> MTENIEAVMSDFWSNPADHFRPNLKALTLYAERQHYVDRWLHVKERWLAPWYLPWWSPLFQLGTWYSQRSRNLFLVENHLSYRPYKFRRNDEDRNNP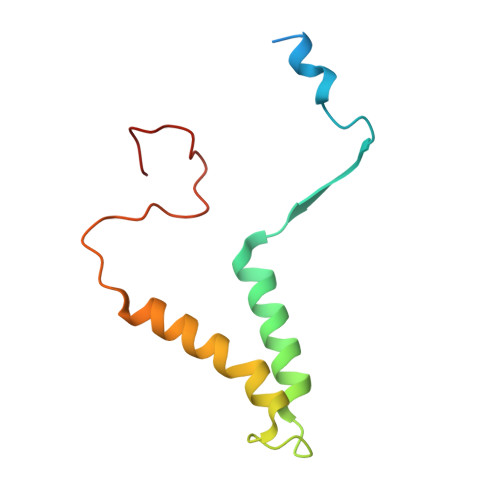Y> AKAI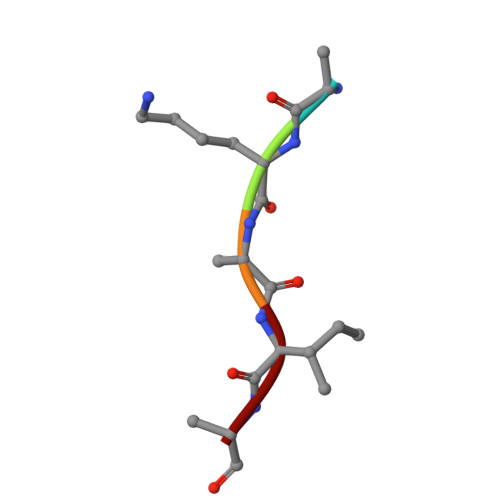A>GGGMLTLIQGKKIVNHLRSRLAFEYNGQLIKILSKNIVAVGSLRREEKMLNDVDLLIIVPEKKLLKHVLPNIRIKGLSFSVKVCGERKCVLFIEWEKKTYQLDLFTALAEEKPYAIFHFTGPVSYLIRIRAALKKKNYKLNQYGLFKNQTLVPLKITTEKELIKELGFTYRIPKKRL[4x]

To provide a molecular basis for designing better drugs targeting polymerases, African swine fever virus DNA Polymerase X (Pol X) was used as a model for the study. As the simplest DNA polymerase identified to date, Pol X belongs to the polymerase X family and is constituted of 174 amino acids. In this chemical reaction, metal-ion A (MeA) is a catalytic ion and decreases the pKa of 3′-OH, facilitating its attack on the α-phosphate of the incoming dNTP, and metal-ion B (MeB) stabilizes the dNTP-DNA-polymerase complex and increases the electrophilicity of the phosphorus center. To clearly understand the phosphodiester-bond-formation mechanism and the metal-ion catalysis of polymerases, we designed modified dNTP substrates with a chiral α-phosphorus center (α-P center) using a single selenium atom, without affecting the overall and local structures, to explore the absolute configuration inversion and probe the mechanisms of the metal ion–oxygen interactions.

In contrast, when using DNA-II (with 3′-OH) and dNTP (dGTP, dGTPαSe-I, or dGTPαSe-II), the DNA extension reaction took place to form DNApost, and the phosphodiester bond was formed (the after-reaction state, with the bond formation), followed by solving the absolute configuration of the Se-atom-modified P-center on DNApost in the product complex (the product-template–polymerase complex: nat-dG_pro, dGSe-I_pro, or dGSe-II_pro). The 3′-OH attacked the incoming dGTP or dGTPαSe diastereomers in the crystallization conditions, thereby generating DNApost and forming the native and Se-modified product complexes. Similarly, the Se-modified product complex (formed from dGTPαSe-Sp) generated extra and very strong electron density only for the Se atom on the P-center, revealing its Rp configuration and indicating the two-metal O coordination. Further, the configurations of polymerization products (using dGTPαSe-I and dGTPαSe-II) were determined as Sp and Rp, respectively. Based on these structural observations, the Se-modified P-center configurations on the two dGSe_pro structures (synthesized from dGTPαSe-Rp and -Sp) were determined as Sp and Rp, respectively, indicating the P-center inversion. Though one nat-dG_pro complex and two dGSe_pro complexes belonged to P212121 and P21 space groups, respectively, their structures with the polymerase were virtually identical, especially the two dGSe_pro structures (RMSD: 0.2 Å). In addition, the complex structures of the three products generated from the native and Se-modified dGTPs were virtually identical, and the absolute configurations of the Se-generated P-centers on the two dGSe_pro complexes from dGTPαSe-Rp and -Sp were determined as Sp and Rp, respectively.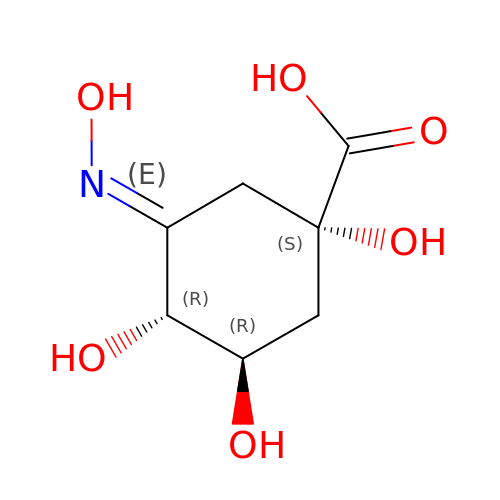3-HYDROXYIMINO QUINIC ACID | C7 H11 N O6 | WASIBXJFRXJWAR-GKQOBJDDSA-N> APKDNHHHHHHANKEATRNAAALFSVDYKAFLNEVANLNKRMGDLRDINGEAGAWARIMSGTGSASGGFSDNYTHVQVGVDKKH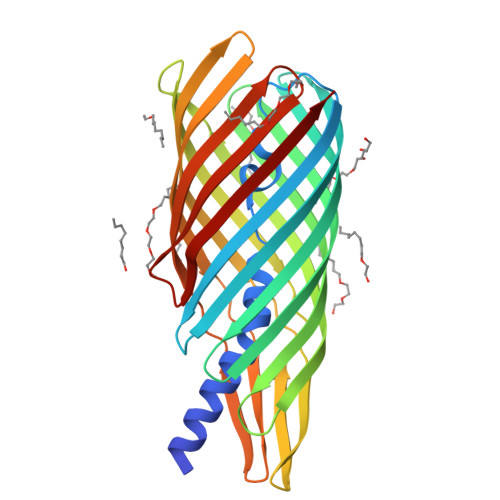ELDGLDLFTGFTVTHTDSSASADVFSGKTKSVGAGLYASAMFDSGAYIDLIGKYVHHDNEYTATFAGLGTRDYSTHSWYAGAEAGYRYHVTEDAWIEPQAELVYGSVSGKQFAWKDQGMHLSMKDKDYNPLIGRTGVDVGKSFSGKDWKVTARAGLGYQFDLLANGETVLRDASGEKRIKGEKDSRMLMSVGLNAEIRDNVRFGLEFEKSAFGKYNVDNAVNANFRYSF>[10x]MPGSIPLIGERFPEMEVTTDHGVIKLPDHYVSQGKWFVLFSHPADFTPVSTTEFVSFARRYEDFQRLGVDLIGLSVDSVCSHIKWKEWIERHIGVRIPFPIIADPQGTVARRLGLLHAESATHTVRGVFIVDARGVIRTMLYYPMELGRLVDEILRIVKAL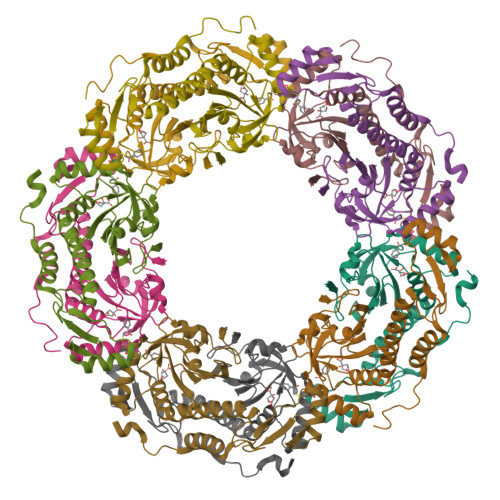KLGDSLKRAVPADWPNNEIIGEGLIVPPPTTEDQARARMESGQYRSLDWWFSWDTPASRDDVEEARRYLRRAAEKPAKLLYEEARTHLH> GHMIKYYNINGQQVPVENATLHVSDLSILRGYGIFDYFLAREGHPLFLDDYLNRFYRSAAELYLEIPFDKAELRRQIYALLQANEVREAGIRLVLTGGYSPDGYTPVNPNLLIMMYDLPASAWEFSAQGIKIITHPFQRELPEVKTINYSTGIRMLKTIKERGATDLIYVDQGEWIRESARSNFFLVMPDNTIVTADEKILWGITRRQVIDAAREAGYAVEERRIHITELDQAREAFFTSTIKGVMAIGQIDDRVFGDGTIGKVTQELQDLFVGKVKAYLETC

Pyridoxal 5’-phosphate (PLP)-dependent transaminases (aminotransferases, TAs, EC [2.6.1.X]) catalyze the transfer of an amino group from amino acid or amine to keto acid or ketone to form a new amino acid/amine and keto acid/ketone. TA_Halhy belongs to the group of fold type IV transaminases and efficiently catalyzes transamination reactions between D-amino acids and α-keto acids; specific activity in the reaction between D-glutamate and pyruvate in 50 mM potassium phosphate buffer (pH 8.0) hits the record high values for TAs: 380 ± 10 μmol/min per mg of protein at 40°C. The structure of this enzyme, dimer being its functional unit, has been identified. Like for the studied fold type IV TAs, the active site of TA_Halhy can be subdivided into two parts (the O- and P-pockets); the amino acid residues of these pockets are involved in substrate binding, thus being responsible for the stereospecificity of catalytic transformation. TA_Halhy stands out among the known fold type IV TAs by featuring four positively charged functional groups in its active site (side groups of amino acids Arg28*, Arg90, Arg179, and Lys241).

3-Aminooxypropionic acid was shown to interact with PLP in the active site of TA_Halhy to form an oxime that mimics the external aldimine of PLP and D-glutamic acid; therefore, successful crystallization and solving the complex’s structure make it possible to identify the functional groups involved in the binding of this specific substrate. We successfully crystallized the TA_Halhy complex with the oxime of PLP and 3-aminooxypropionic acid in the active site. The structures of the holoenzyme and complex with the oxime are well-superposed (RMSD for Cα atoms is 0.31). Differences are mostly observed for the positions of loops. Importantly, the carboxyl group of the oxime of PLP and 3-aminooxypropinic acid is located in the O-pocket, although in fold type IV D-amino acid transaminases the side group of the substrate binds within the P-pocket, while the O-pocket binds the α-carboxyl group of substrates (D-amino acid or keto acid), which forms hydrogen bonds with the functional groups of the active site. In the resulting structure, the carboxyl group of the oxime forms hydrogen bonds with the guanidine groups of Arg28* and Arg179 residues. The Arg90 and Lys241 residues are not involved in the binding of the carboxyl group; the side group positions in all the aforementioned residues remain unchanged. The observed adduct position in the active site of TA_Halhy mimics substrate inhibition rather than the formation of an external aldimine with D-glutamic acid as a specific substrate.> SGHHEHST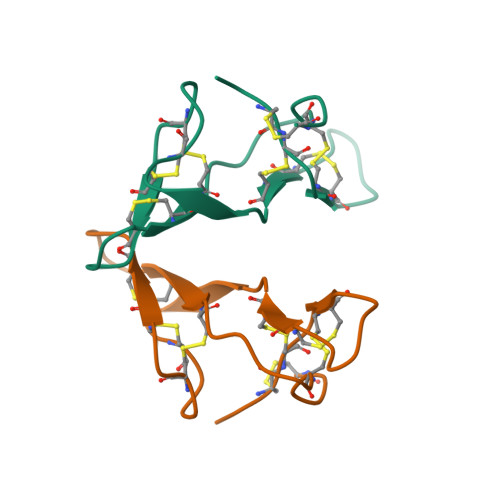DZPSZSSKPCCDHCSCTKSIPPQCRCTDLRLDSCHSACKSCICTLSIPAQCVCDDIDDFCYEPCKSSHSDDDNNN> SDFYLPGDYLLGGLFSLHANMKGIVHLNFLQVPMCKEYEVKVIGYNLMQAMRFAVEEINNDSSLLPGVLLGYEIVDVCYISNNVQPVLYFLAHEDNLLPIQEDYSNYSSRVVAVIGPDNSESVMTVANFLSLFLLPQITYSAISDELRDKVRFPALLRTTPSADHHIEAMVQLMLHFRWNWIIVLVSNDTYGRDNGQLLGERVARRGICIAFQETLPTLQPNQNMTSEERQRLVTIVDKLQQSTARVVVVFSPDLTLYHFFNEVLRQNFTGAVWIASESWAIDPVLHNLTELRHLGTFLGITIQSVPIPGFSEFREWGPQAGPPPLSRTSQSYTCNQECDNCLNATLSFNTILRLSGERVVYSVYSAVYAVAHALHSLLGCDKSTCTKRVVYPWQLLEEIWKVNFTLLDHQIFFDPQGDVALHLEIVQWQWDRSQNPFQSVASYYPLQRQLKNIQDISWHTINNTIPMSMCSKRCQSGQKKKPVGIHVCCFECIDCLPGTFLNHTEDEYECQACPNNEWSYQSETSCFKRQ;> LCLSQQFKAQGDYILGGLFPLGSTEEATLNQRTQPNSIPCNRFSPLGLFLAMAMKMAVEEINNGSALLPGLRLGYDLFDTCSEPVVTMKSSLMFLAKVGSQSIAAYCNYTQYQPRVLAVIGPHSSELALITGKFFSFFLMPQVSYSASMDRLSDRETFPSFFRTVPSDRVQLQAVVTLLQNFSWNWVAALGSDDDYGREGLSIFSSLANARGICIAHEGLVPQHDTSGQQLGKVLDVLRQVNQSKVQVVVLFASARAVYSLFSYSIHHGLSPKVWVASESWLTSDLVMTLPNIARVGTVLGFLQRGALLPEFSHYVETHLALAADPAFCASLNAELDLEEHVMGQRCPRCDDIMLQNLSSGLLQNLSAGQLHHQIFATYAAVYSVAQALHNTLQCNVSHCHVSEHVLPWQLLENMYNMSFHARDLTLQFDAEGNVDMEYDLKMWVWQSPTPVLHTVGTFNGTLQLQQSKMYWPGNQVPVSQCSRQCKDGQVRRVKGFHSCCYDCVDCKAGSYRKHPDDFTCTPCNQDQWSPEKSTACLP

Sugars and other sweet-tasting compounds are detected by the sweet taste receptor, a member of the class C GPCR family. The sweet receptor is a heterodimer composed of TAS1R2 and TAS1R3,3,4 two type 1 taste receptor family members that share the distinctive architecture of class C GPCRs: a large extracellular Venus flytrap (VFT) domain, responsible for ligand recognition; a cysteine-rich domain (CRD); and a seven-transmembrane (7TM) domain that mediates G protein coupling. To address this gap, here we present cryo-electron microscopy (cryo-EM) structures of the sweet receptor in the inactive, unliganded state, as well as in the activated, sucralose- and advantame-bound states. Unlike other class C GPCRs, such as mGluR, CaSR and GABAB receptors, where agonists stabilize inter-subunit VFT interactions to promote activation, the sweet receptor is activated by the rearrangement of a TAS1R2 VFT loop, which destabilizes interactions between the lower VFT lobes and the VFT–CRD interfaces.

In the presence of sweeteners, the human/mouse sweet receptor adopts two distinct conformations, which we refer to as compact and loose. In the compact conformation, the VFT LB2s remain packed; in the loose conformation, LB2s of the two subunits disengage. In the presence of sucralose, we observed a prominent ligand density in the TAS1R2 VFT domain, consistent with previous functional studies showing that sucralose binds exclusively to TAS1R2.3,12 The VFT LB1 and LB2 form a clamshell-like structure, and sucralose adopts a U-shape that fits snugly within the cleft between the lobes. Its chlorinated fructose and glucose rings are oriented nearly side by side, in a vertical arrangement, allowing multiple polar interactions with residues lining the interlobe pocket: the chlorine interacts with Asn143; the hydroxyl and chlorine groups participate in a H-bonding network with polar residues including Asp142, Asp278, and Glu302. Compared to the apo state, sucralose binding induces closure of the TAS1R2 VFT clamshell, with the bottom of LB2 lifting by up to 7 Å, reducing the clamshell opening from 112° (apo) to 105° (compact) and further to 103° (loose). Thus, the loose state shows the highest degree of TAS1R2 VFT closure, whereas the compact state may correspond to an intermediate along the activation trajectory. The closure of the TAS1R2 VFT clamshell induced by sweetener binding leads to the formation of salt bridges between LB1 Lys65 and LB2 Asp278, which are brought into proximity in the compact state and engage further to form stable interactions in the loose state. In addition, a loop in TAS1R2 VFT LB1 (around residues 45–57), which is disordered in the apo and compact states, becomes ordered in the loose state and inserts into the interface between TAS1R2 and TAS1R3. It interacts with the region surrounding Tyr131 and Phe159 of TAS1R3, pushing against an adjacent loop near Thr179, which is displaced by ~2 Å.>MSSRKELANAI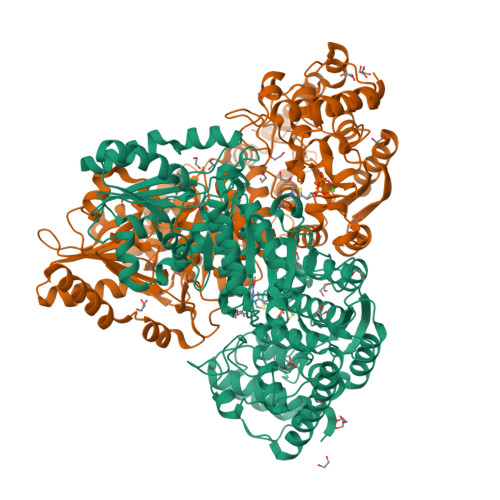RALSMDAVQKAKSGHPGAPMGMADIAEVLWRDFLKHNPQNPSWADRDRFVLSNGHGSMLIYSLLHLTGYDLPMEELKNFRQLHSKTPGHPEVGYTAGVETTTGPLGQGIANAVGMAIAEKTLAAQFNRPGHDIVDHYTYAFMGDGCMMEGISHEVCSLAGTLKLGKLIAFYDDNGISIDGHVEGWFTDDTAMRFEAYGWHVIRDIDGHDAASIKRAVEEARAVTDKPSLLMCKTIIGFGSPNKAGTHDSHGAPLGDAEIALTREQLGWKYAPFEIPSEIYAQWDAKEAGQAKESAWNEKFAAYAKAYPQEAAEFTRRMKGEMPSDFDAKAKEFIAKLQANPAKIASRKASQNAIEAFGPLLPEFLGGSADLAPSNLTLWSGSKAINEDAAGNYIHYGVREFGMTAIANGISLHGGFLPYTSTFLMFVEYARNAVRMAALMKQRQVMVYTHDSIGLGEDGPTHQPVEQVASLRVTPNMSTWRPCDQVESAVAWKYGVERQDGPTALILSRQNLAQQERTEEQLANIARGGYVLKDCAGQPELIFIATGSEVELAVAAYEKLTAEGVKARVVSMPSTDAFDKQDAAYRESVLPKAVTARVAVEAGIADYWYKYVGLNGAIVGMTTFGESAPAELLFEEFGFTVDNVVAKAKELLHHHHHH[2x]Prostate-specific membrane antigen (PSMA), also known as glutamate carboxypeptidase II (GCPII), folate hydrolase (FOLH1), or N-acetylated α-linked acidic dipeptidase (NAALADase), is a membrane-bound metallopeptidase, featuring two zinc ions in its active site. Importantly, the PSMA is overexpressed on prostate cancer cells and the enzyme thus attracts significant attention as a target for the delivery of imaging and therapeutic agents and continues to serve as an important biomarker of prostate cancer. To identify molecular mechanisms behind markedly different potencies of bisubstituted sulfamides and phosphinates/phosphonates, we solved X-ray structures of complexes between PSMA, a well-studied bimetallic metallopeptidase, and sulfamide-based inhibitors. Structural data showed that while monosubstituted sulfamides coordinate active-site zinc ions via the free negatively charged amino group in a canonical manner, their bisubstituted counterparts adopt an atypical binding pattern divergent from expected positioning of corresponding tetrahedral reaction intermediates.

The N1 functionalization of 9 has a significant negative impact on the inhibition potency, resulting in IC50 values of 103 and 165 μM for 3 and 4, respectively. The use of the hydrolytically inactive PSMA(E424M) mutant was required due to the fact that upon cocrystallization of 3 and 4 with the wild-type enzyme, the inhibitors were hydrolyzed and only the hydrolytic products were observed in the PSMA active site (data not shown). Similar to the PSMA/9 complex, the P1′ glutamates of 3 and 4 are well-defined in the Fo-Fc difference map and they occupy overlapping canonical positions within the S1′ pocket. Interestingly, the placement of the sulfamide functionality differs between the two compounds. In the PSMA/4 complex, the sulfamide function is rotated by 120 degrees. Consequently, the positioning and interaction pattern of the first sulfamide oxygen is identical to that of 3, while the second oxygen atom is rotated to the position of the P1 nitrogen atom of 4, where it is hydrogen-bonded to the catalytic water/OH– (2.7 Å), Asn519 (3.1 Å), and Asp453 (3.2 Å), and at a distance of 3.4 Å from the cocatalytic zinc ion. Finally, the β-carboxylate group of 3 forms ion pairs and the hydrogen bond with Arg536 (3.0 and 3.3 Å) and Ser454 (2.5 Å), respectively, while the γ-carboxylate of 4 is disordered in the structure pointing toward its positional flexibility and the absence of strong interactions with residues of the enzyme. At the same time, given the expected conformational flexibility of 4 in the crystal structure (as witnessed by the weak Fo-Fc peaks for the P1 moiety of the inhibitor), such a rearrangement can be plausible.

> KSSNEATNITPKHNMKAFLDELKAENIKKFLYNFTQIPHLAGTEQNFQLAKQIQSQWKEFGLDSVELAHYDVLLSYPNKTHPNYISIINEDGNEIFNTSLFEPPPPGYENVSDIVPPFSAFSPQGMPEGDLVYVNYARTEDFFKLERDMKINCSGKIVIARYGKVFRGNKVKNAQLAGAKGVILYSDPADYFAPGVKSYPDGWNLPGGGVQRGNILNLNGAGDPLTPGYPANEYAYRRGIAEAVGLPSIPVHPIGYYDAQKLLEKMGGSAPPDSSWRGSLKVPYNVGPGFTGNFSTQKVKMHIHSTNEVTRIYNVIGTLRGAVEPDRYVILGGHRDSWVFGGIDPQSGAAVVHEIVRSFGTLKKEGWRPRRTILFASWDAMEFGLLGSTEWAEENSRLLQERGVAYINADSSIEGNYTLRVDCTPLMYSLVHNLTKELKSPDEGFEGKSLYESWTKKSPSPEFSGMPRISKLGSGNDFEVFFQRLGIASGRARYTKNWETNKFSGYPLYHSVYETYELVEKFYDPMFKYHLTVAQVRGGMVFELANSIVLPFDCRDYAVVLRKYADKIYSISMKHPQEMKTYSVSFDSLFSAVKNFTEIASKFSERLQDFDKSNPIVLRMMNDQLMFLERAFIDPLGLPDRPFYRHVIYAPSSHNKYAGESFPGIYDALFDIESKVDPSKAWGEVKRQIYVAAFTVQAAAETLSEVA>[2x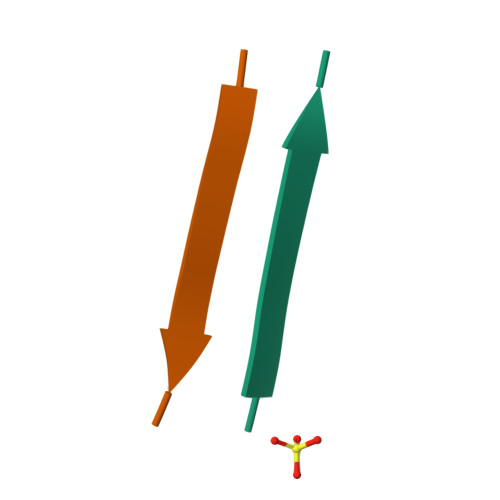]NFLVHSS>[2x]SVVLPVAKRGEDILKLIAAPVSANELNSNWLYQLADAMHATMLERNGVGIAAPQVYISKRVIIVASRPNPRYPDAPEMNAVVMVNPEILEFSSEMCLGEEGCLSVPDERGQVERAE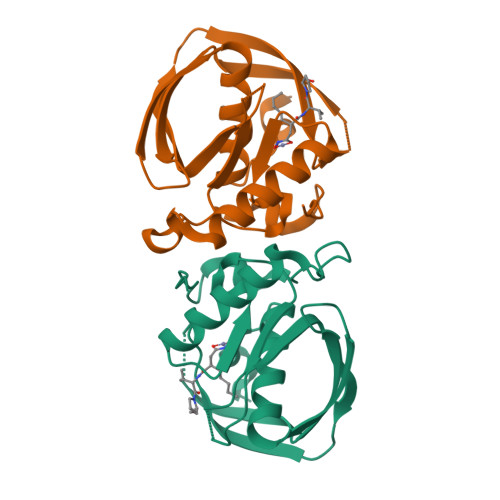MVKVKYLTLQGEMVETVFQGFPARIVQHEVDHLNGILFVERIS2,4-dimethoxyphenol | C8 H10 O3 | 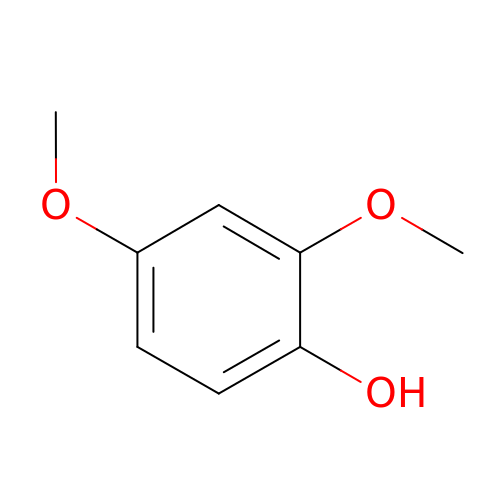MNVMYTVDDOXZLS-UHFFFAOYSA-N>[6x]MSRDRFRSRGGGGGGFHRRGGGGGRGGLHDFRSPPPGMGLNQNRGPMGPGPGGPKPPIPPPPPHQQQPQQPPPQQPPPQQPPPHQQPPPHQPPHQQPPPPPQDSSKPVVPQGPGSAPGVSPAPPPAGSAPPANPPTTGAPPGPGPTPTPPPAVTSATPGPPPPSTPSSGVSTTPPQSGGPPPPPAGGAGPGPKQGPGPGPGGPKGGKMPGGPKPGGGPGMGAPGGHPKPPHRGGGEPRGGRQHHPPYHQQHHQGPPPGGPAARTEEKISDSEGFKANLSLLRRPGEKTYTQRCRLFVGNLPADITEDEFKRLFAKYGEPGEVFINKGKGFGFIKLESRALAEIAKAELDDTPMRGRQLRVRFATHAAALSVRNLSPYVSNELLEEAFSQFGPIERAVVIVDDRGRSTGKGIVEFASKPAARKAFERCSEGVFLLTTTPRPVIVE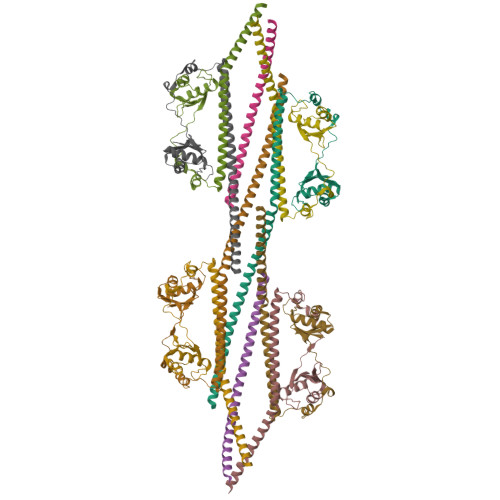PLEQLDDEDGLPEKLAQKNPMYQKERETPPRFAQHGTFEYEYSQRWKSLDEMEKQQREQVEKNMKDAKDKLESEMEDAYHEHQANLLRQDLMRRQEELRRMEELHSQEMQKRKEMQLRQEEERRRREEEMMIRQREMEEQMRRQREESYSRMGYMDPRERDMRMGGGGTMNMGDPYGSGGQKFPPLGGGGGIGYEANPGVPPATMSGSMMGSDMRTERFGQGGAGPVGGQGPRGMGPGTPAGYGRGREEYEGPNKKPRF;>MQSNKTFNLEKQNHTPRKHHQHHHQQHHQQQQQQQQQPPPPIPANGQQASSQNEGLTIDLKNFRKPGEKTFTQRSRLFVGNLPPDITEEEMRKLFEKYGKAGEVFIHKDKGFGFIRLETRTLAEIAKVELDNMPLRGKQLRVRFACHSASLTVRNLPQYVSNELLEEAFSVFGQVERAVVIVDDRGRPSGKGIVEFSGKPAARKALDRCSEGSFLLTTFPRPVTVEPMDQLDDEEGLPEKLVIKNQQFHKEREQPPRFAQPGSFEYEYAMRWKALIEMEKQQQDQVDRNIKEAREKLEMEMEAARHEHQVMLMRQDLMRRQEELRRMEELHNQEVQKRKQLELRQEEERRRREEEMRRQQEEMMRRQQEGFKGTFPDAREQEIRMGQMAMGGAMGINNRGAMPPAPVPTGTPAPPGPATMMPDGTLGLTPPTTERFGQAATMEGIGAIGGTPPAFNRPAPGADFAPNKRRRY[4x]>GIPKTGGDKSVINLKFILAAIDAHKKLGWEPAGSKRIGFDVADDGEDANATTLMHGNVIMEVDEWDGLEDELLKSSSRVY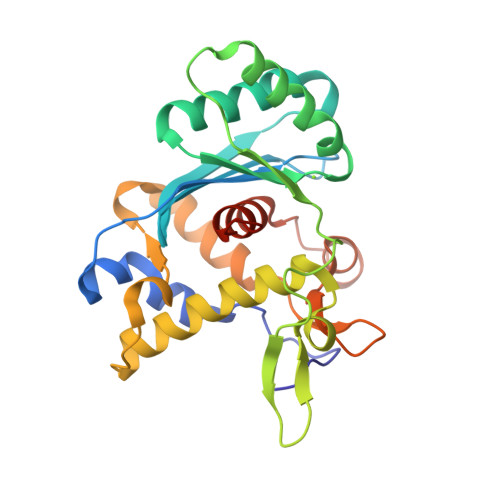NLAKIKGASVTYDSIGVGAHVGSKFAELNDASPDFKLIYDPFNAGGAVDKPDDVYMKLPHTTIKNKDHFSNIKAQKWEEVATRFRKTYEAVEHGKVYPFDELISINSETIHPDKLNQLCIELSSPRKDLDMNGRFKVESKKDMREKRKIKSPNIADSVIMSAILPIRKPKGFFDF[2x]>GPGAYISLNYHSPTIGMHQNLTVILPEDQSFFNSDTTVKPLKTLMLLHGLSSDETTYMRYTSIERYANEHKLAVIMPNVDHSAYANMAYGHSYYDYILEVYDYVHQI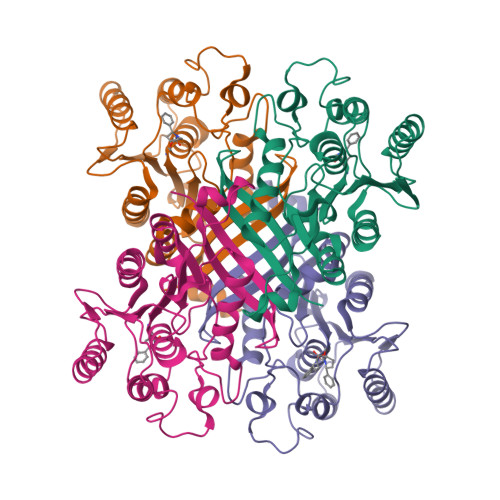FPLSKKRDDNFIAGHSMGGYGTIKFALTQGDKFAKAVPLSAVFEAQNLMDLEWNDFSKEAIIGNLSSVKGTEHDPYYLLDKAVAEDKQIPKLLIMCGKQDFLYQDNLDFIDYLSRINVPYQFEDGPGDHDYAYWDQAIKRAITWMVND[4x]>[4x]METKEIFDAAPLSVSQFLSETGQGLYIPPYQRAYS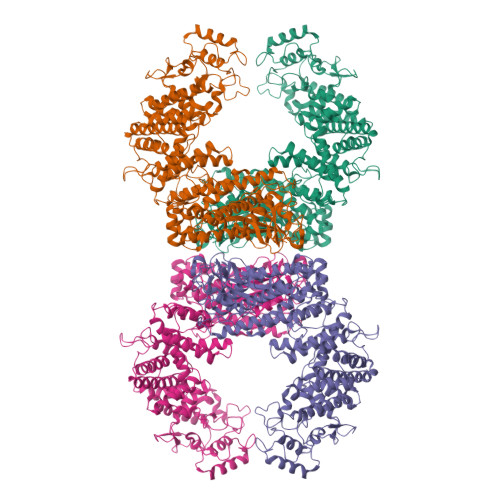WELPKIRRLLSDVAHGLDQLAEFEDSICFLGTVIALRDINYTTVEPKYRSQVPSKVMTIIDGQQRMTTLLLLTTVLHEEIRVRAEKLTRDDEPSVWCYNQALDVTGRLSNCFEEDMRYGEHRYYPRLIRSYYDVWSRNKGEARYRSPIGYYLESYGAYARDPDAVKPYRHVPIDPDKTDGVDLEAYRHLDRMRDQMRSMLRKAVGAGVKREDDIQLPTGTDIGQSQNLQFALFNSEFPPSVVEQLEDDAKMTPLTRLIVFANYLLHRVTVAVVTAKREDYGFDMFEALNTTGQPLTAIETFKPRAIKEEGLDEWQESESKLHFDVVEAYLDREGSSSADKRQTVTSSVLLPFAMFQDGTKLTKRLNDQRRYLRTVFDKDPDIVARRKVLAGLAQVARFYEGPWGSPTKVPSCDDATLRTQAGIALAALREGGHDIVVGLLTRYFAAHRLSSPETVESSARQFLLAARSCAAFYALWRGSFGSTAGIDGVYRSLMTHVVEEGMPRFARFERDLTEVPPVEALQSYLKEQLRSEGIYDKQQWVARAAMTPVYQHSKPLTRLLLLAASQNSTPDSATPGLVVRGKSGLLETLELERWNDEAFATIEHVAPQAPSSNGSWNADLYEDPELINRIGNLTLLPAVENASASNRAWHLKRLMFRALSAATVEEAEKTLADAEAQGLRLGSGAGEIVRQARYLPLVAALAQREEEWTAEFVEARSQRLCSLAWDALTPWLGFEP> MAHAGRTGYDNREIVMKYIHYKLSQRGYEWDAGDDVEE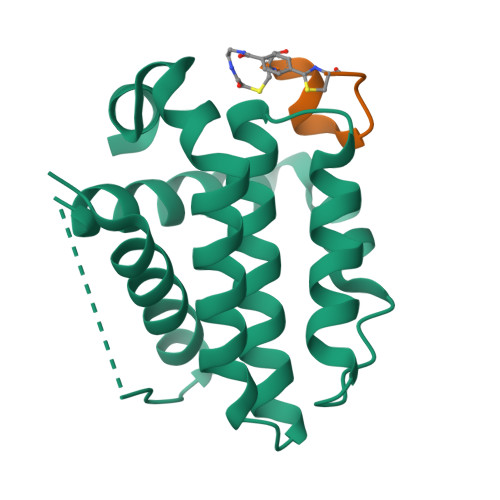NRTEAPEGTESEVVHLTLRQAVDDFSRRYRRDFAEMSSQLHLTPFTARGRFATVVEELFRDGVNWGRIVAFFEFGGVMCVESVNREMSPLVDNIALWMTEYLNRHLHTWIQDNGGWDAFVELYGPSMR;> CPARYGWDYECX>MSLKQSKRILVVDDDQAMAAAIERVLKRDHWQVEIAHNGFDAGIKLSTFEPAIMTLDLSMPKLDGLDVIRSLRQNKVANQPKILVVSGLDKAKLQQAVTEGADDYLEKPFDNDALLDRIHDLVNEGHHHHHH[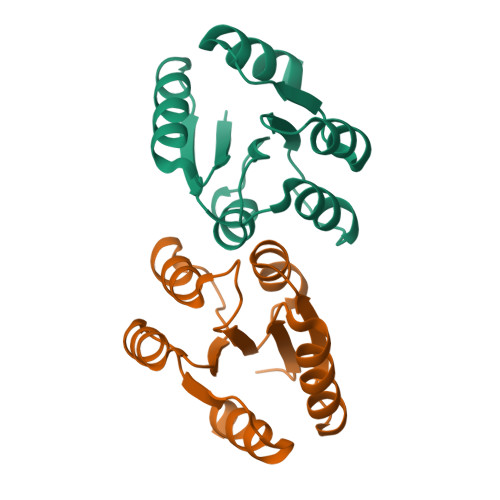24x]>[4x]GSGSTRDYEIQRERIELGRCIGEGQ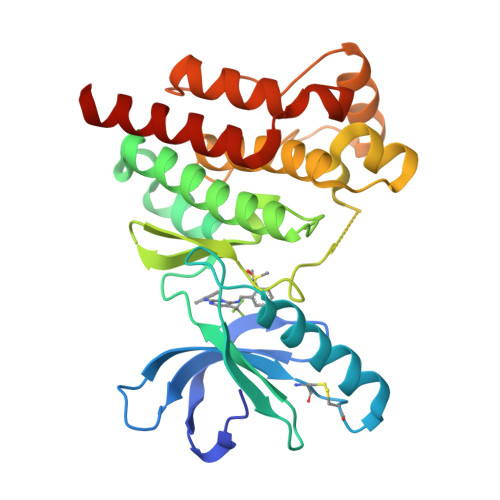FGDVHQGIYMSPENPALAVAIKTCKNCTSDSVREKFLQEALTMRQFDHPHIVKLIGVITENPVWIIMELCTLGELRSFLQVRKYSLDLASLILYAYQLSTALAYLESKRFVHRDIAARNVLVSSNDCVKLGDFGLSRYMEDSTYYKASKGKLPIKWMAPESINFRRFTSASDVWMFGVCMWEILMHGVKPFQGVKNNDVIGRIENGERLPMPPNCPPTLYSLMTKCWAYDPSRRPRFTELKAQLSTILEEEKAQQEE>MKAFILAAGSGERLEPITHTRPKAFVPILSKPLIEYQIEYLRKCGIRDITVIVSSKNKEYFEKKLKEISIVTQKDDIKGTGAAILSAKFNDEALIINGDLFFSNEKEICNIITLKENAIIGVKVSNPKDYGVLVLDNQNNLSKIIEKPEIPPSNLINAGIYKLNSDIFTYLDKISISERGELELTDAINLMAKDHRVKVIEYEGYWMDIGKPWNIIDVNKWALDNLVFSQNLGNVEDNVKIKGKVIIEEDAEIKSGTYIEGPVYIGKGSEIGPNSYLRPYTILVEKNKIGASVEVKESVIMEGSKIPHLSYVGDSV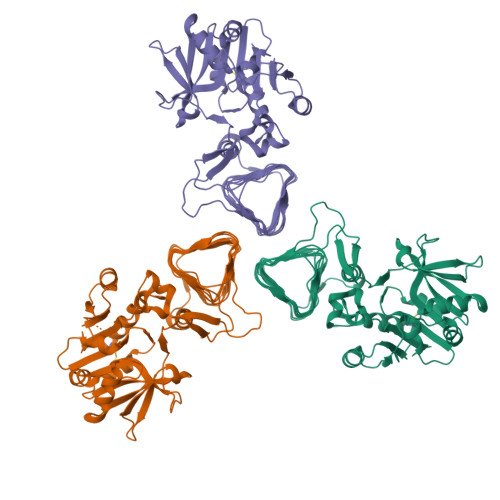IAEDVNFGAGTLIANLRFDEKEVKVNVKGKRISSGRRKLGAFIGGHVRTGINVTILPGVKIGAYARIYPGAVVNRDVGYGEFFKVLEHHHHHH[6x]> IREILKMGDERLLRIAQPVPSELLGSEELQ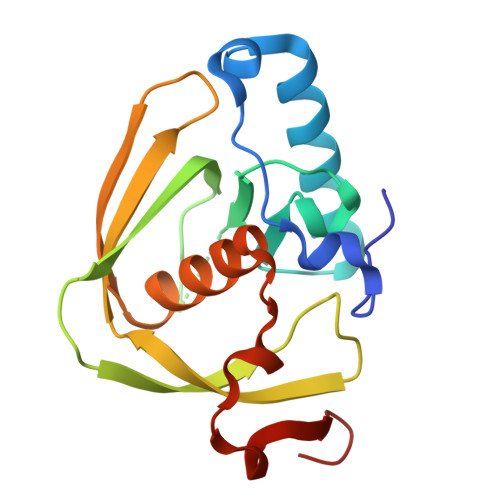RLIDDMFETMHHVGGVGLAAPQIGVDLQLVIFGFERSERYPDAPAVPPTILLNPRITPLDDEMEEGWEGCLSVPGLRGAVSRHRRIRYQGLDPQGQPIDRSVEGFHARVVQHECDHLIGRLYPSRITDFSKFGFTEVLFP>MKILITGGAGFIGSAVVRHIIKNTQDTVVNIDKLTYAGNLESLSDISESNRYNFEHADICDSAEITRIFEQYQPDAVMHLAAESHVDRSITGPAAFIETNIVGTYALLEVARKYWSALGEDKKNNFRFHHISTDEVYGDLPHPDEVENSVTLPLFTETTAYAPSSPYSASKASSDHLVRAWRRTYGLPTIVTNCSNNYGPYHFPEKLIPLVILNALEGKPLPIYGKGDQIRDWLYVEDHARALHMVV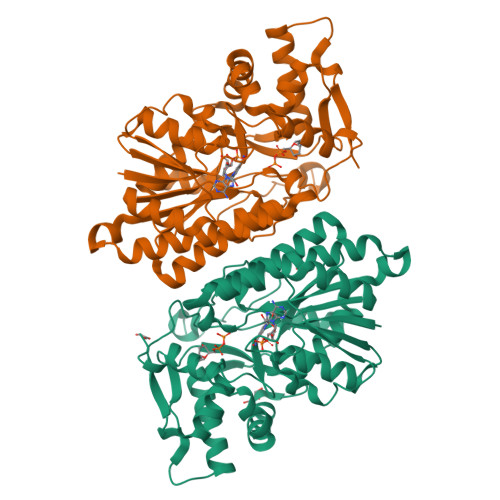TEGKAGETYNIGGHNEKKNLDVVFTICDLLDEIVPKATSYREQITYVADRPGHDRRYAIDAGKISRELGWKPLETFESGIRKTVEWYLANTQWVNNVKSGAYQSWIEQNYEGRQ[2x]> MLHAVRLLSCWRPAAIQHLPDVAPXAPVQEVEKSHARYRPLSLRARQTLSEKSDDLQYHVVTQEWFGERVDSFLTCHYPQWDYETIKRLVQQGHIYRYRKNGKKKFTRLTDRLEFD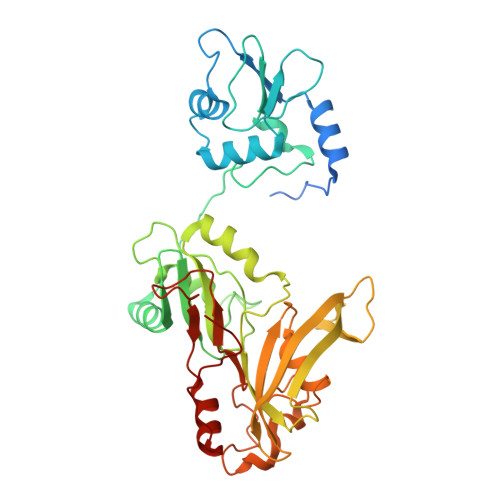ELLVVPTRAFWEKQLAPPSGVLEETDGPKFKLSATAREMAHNMVLFKNEHVIVINKPHGLPMMPTDDPQEMSIAAMLPAWKFTNVAKPVVCHNLDRETSGCVVLARTRNAHRMLGRMFVKRVVPNSVYWSFCVGKPTVNYGRVRMHFDITRGNKGDIIVARPSPTKTSKVAIAEFVVNASALEFGSFISFYPLTTRRHQERIMAAHALRCPVLGDAKYGGDAAFPSSLSLFWDPENKGLPLHLHHRKIQLPYKNTAGEFICVTAPLPTQMEKTFKKLGWPCEVDDPLIPG>[2x]MGRKIVFFDIDGTLLDEQKQLPLSTIEAVRRLKQSGVYVAIATGRAPFMFEHVRKQLGIDSFVSFNGQYVVFEGNVLYKQPLRREKVRALTEEAHKNGHPLVFMDAEKMRASIGDHPHIHVSMASLKFAHPPVDPLYYENKDIYQ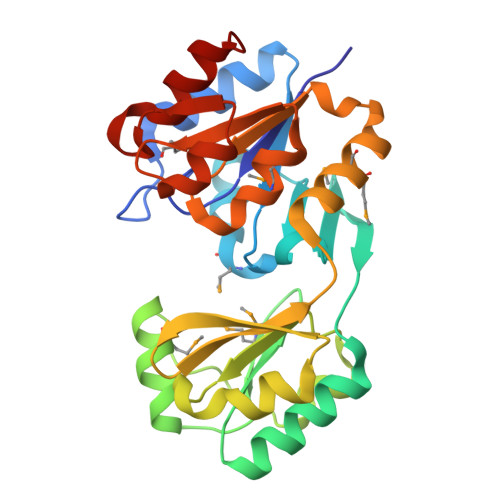ALLFCRAEEEEPYVRNYPEFRFVRWHDVSTDVLPAGGSKAEGIRMMIEKLGIDKKDVYAFGDGLNDIEMLSFVGTGVAMGNAHEEVKRVADFVTKPVDKEGIWYGLKQLQLIR> GGACUUCG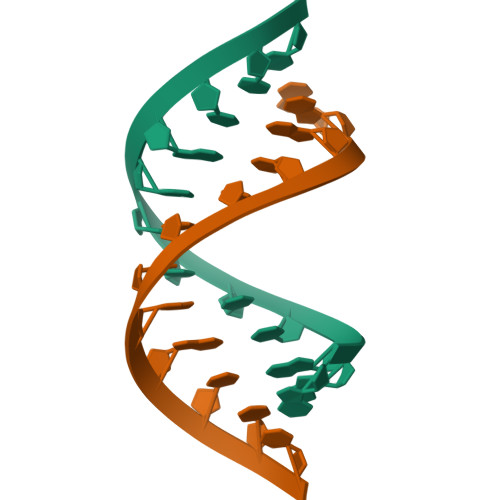GUCC>GHMDDVLRRNPLFAALDDEQSAELRASMSEVTLARGDTLFHEGDPGDRLYVVTEGKVKLHRTSPDGRENMLAVVGPSELIGELSLFDPGPRTATGTALTEVKLLALGHGDLQPWLNVRPEVATA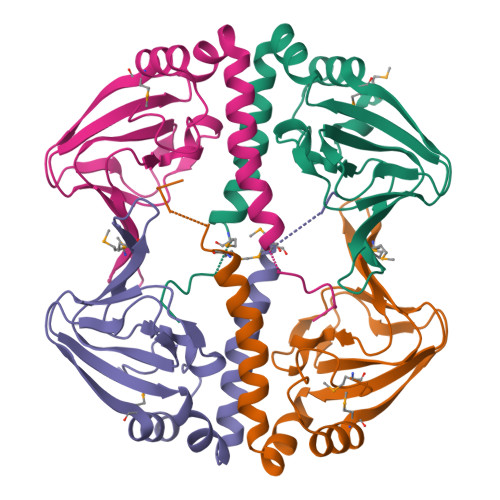LLRAVARRLRKTNDAMSDLVFSDGS[4x]>[14x]MKIQMRNKKVLSFLTLTAIVSQALVYPVYAQTSTSNHSNKKKEIVNEDILPNNGLMGYYFTDEHFKDLKLMAPIKDGNLKFEEKKVDKLLDKDKSDVKSIRWTGRIIPSKDGEYTLSTDRDDVLMQVNTESTISNTLKVNMKKGKEYKVRIE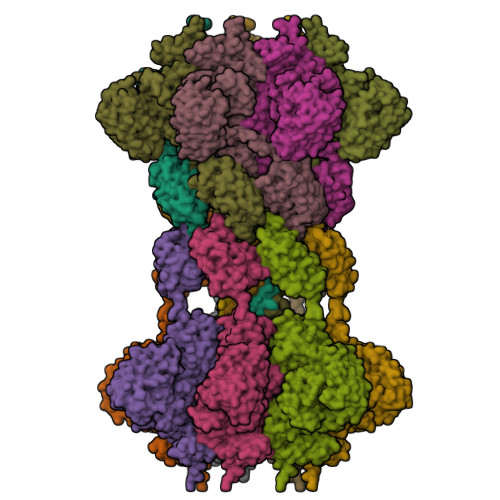LQDKNLGSIDNLSSPNLYWELDGMKKIIPEENLFLRDYSNIEKDDPFIPNNNFFDPKLMSDWEDEDLDTDNDNIPDSYERNGYTIKDLIAVKWEDSFAEQGYKKYVSNYLESNTAGDPYTDYEKASGSFDKAIKTEARDPLVAAYPIVGVGMEKLIISTNEHASTDQGKTVSRATTNSKTESNTAGVSVNVGYQNGFTANVTTNYSHTTDNSTAVQDSNGESWNTGLSINKGESAYINANVRYYNTGTAPMYKVTPTTNLVLDGDTLSTIKAQENQIGNNLSPGDTYPKKGLSPLALNTMDQFSSRLIPINYDQLKKLDAGKQIKLETTQVSGNFGTKNSSGQIVTEGNSWSDYISQIDSISASIILDTENESYERRVTAKNLQDPEDKTPELTIGEAIEKAFGATKKDGLLYFNDIPIDESCVELIFDDNTANKIKDSLKTLSDKKIYNVKLERGMNILIKTPTYFTNFDDYNNYPSTWSNVNTTNQDGLQGSANKLNGETKIKIPMSELKPYKRYVFSGYSKDPLTSNSIIVKIKAKEEKTDYLVPEQGYTKFSYEFETTEKDSSNIEITLIGSGTTYLDNLSITELNSTPEILDEPEVKIPTDQEIMDAHKIYFADLNFNPSTGNTYINGMYFAPTQTNKEALDYIQKYRVEATLQYSGFKDIGTKDKEMRNYLGDPNQPKTNYVNLRSYFTGGENIMTYKKLRIYAITPDDRELLVLSVD> MRVLLIHADYFEYEVKDKALKNPEPISEDMKRGRMEEVLVAFISVEKVDEKNPEEVSLKAIEEISKVAEQVKAENVFVVPWAHLSSELAKPSVAMDILNRV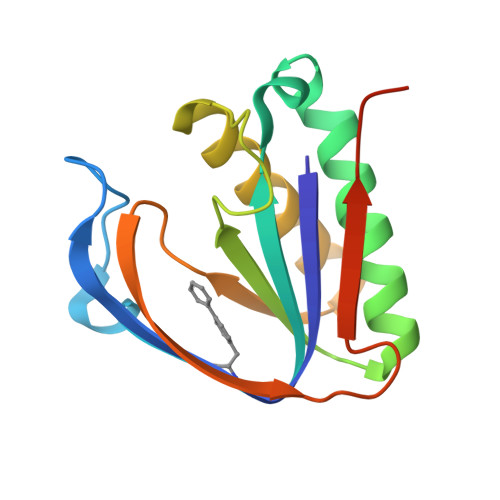YQGLKERGFNVGKAPFGYYIAVKISCKGHPLAELSRTIVPEELEHHHHHH> MKVISLKKDSFNKGGAVITLLPEDKEDLFTVYQIVDKDDELIFKKKFTSKLDEAGKKKSTDLVKLKIKVISEDFDMKDEYLKYKGVTVTDESGASNVDIPVGKYLSFTLDYVYPFTIIKQNFNKFMQKLLNEACNIEYKSDTAAVVLQEGIAHVCLVTSSSTILKQKIEYSMPKKKRTTDVLKFDEKTEKFYKAIYSAMKKDLNFDKLKTIILCSPGFYAKILMDKIFQYAEEEHNKKILDNKGMFFIAHCSTGYLQGINEVLKNPLYASKLQDTKYSKEIMVMDEFLLHLNKDDDKAWYGEKEVVKAAEYGAISYLLLTDKVLHSDNIAQREEYLKLMDSVESNGGKALVLSTLHSLGEELDQLTGIACILKYPLPDLDEDDGEE;> MAYSDYSDGADDMPDFHDEGEFDDYLNDDEYELMNEVFPTLKAQLQDYQGWDNLSLKLALFDNNFDLESTLAELKKTLKKKKTPKKPIAAANGSANVTQKLANISISQQRPNDRLPDWLDEEESEGERNGEEANDEKTVQRYYKTTVPTKPKKPHDISAFVKSALPHLSFVVLGHVDAGKSTLMGRLLYDLNIVNQSQLRKLQRESETMGKSSFKFAWIMDQTNEERERGVTVSICTSHFSTHRANFTIVDAPGHRDFVPNAIMGISQADMAILCVDCSTNAFESGFDLDGQTKEHMLLASSLGIHNLIIAMNKMDNVDWSQQRFEEIKSKLLPYLVDIGFFEDNINWVPISGFSGEGVYKIEYTDEVRQWYNGPNLMSTLENAAFKISKENEGINKDDPFLFSVLEIIPSKKTSNDLALVSGKLESGSIQPGESLTIYPSEQSCIVDKIQVGSQQGQSTNHEETDVAIKGDFVTLKLRKAYPEDIQNGDLAASVDYSSIHSAQCFVLELTTFDMNRPLLPGTPFILFIGVKEQPARIKRLISFIDKGNTASKKKIRHLGSKQRA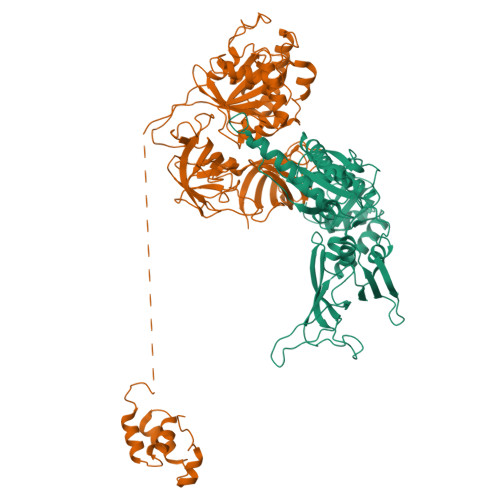FVEIELIEVKRWIPLLTAHENDRLGRVVLRKDGRTIAAGKISEITQ2-(carboxymethyl)-D-aspartic acid | 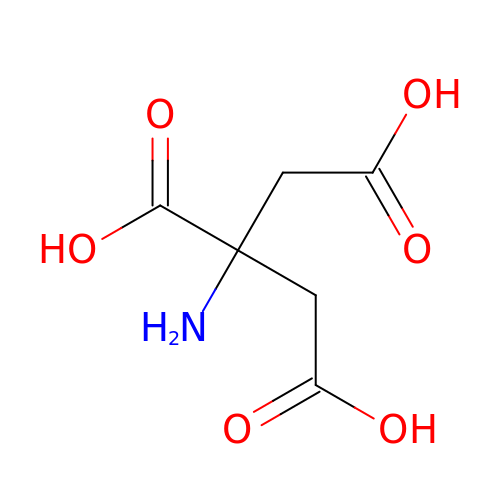C6 H9 N O6 | ZJBWCVAEGNLETQ-UHFFFAOYSA-N> SNGKDVNLEPHLKVTKCLRLFNKQYLLCVQAKLSRPDLKGVTEMIKAKAILYPRKIIGDLPGIDVGHRFFSRAEMCAVGFHNHWLNGIDYMSMEYEKEYSNYKLPLAVSIVMSGQYEDDLDNADTVTYTGQGGHNLTGNKRQIKDQLLERGNLALKHCCEYNVPVRVTRGHNCKSSYTKRVYTYDGLYKVEKFWAQKGVSGFTVYKYRLKRLEGQPELTTDQVNFVAGRIPTSTSEIEGLVCEDISGGLEFKGIPATNRVDDSPVSPTSGFTYIKSLIIEPNVIIPKSSTGCNCRGSCTDSKKCACAKLNGGNFPYVDLNDGRLIESRDVVFECGPHCGCGPKCVNRTSQKRLRFNLEVFRSAKKGWAVRSWEYIPAGSPVCEYIGVVRRTADVDTISDNEYIFEIDCQQTMQGLGGRQRRLRDVAVPMNNGVSQSSEDENAPEFCIDAGSTGNFARFINHSCEPNLFVQCVLSSHQDIRLARVVLFAADNISPMQELTYDYGYALDSVHGPDGKVK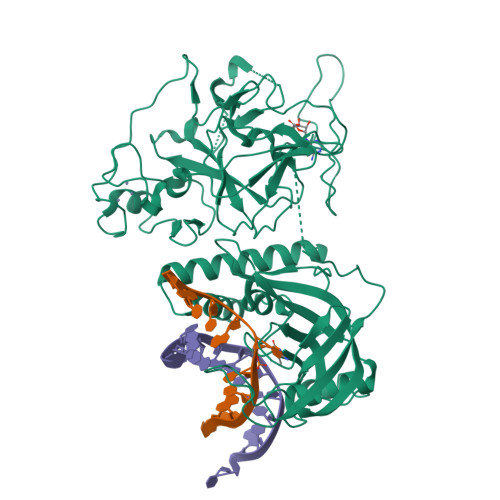QLACYCGALNCRKRLY> MAPVQLENHQLVPPGGGGGGSGGPPSAPAPPPPGAAVAAAAAAAASPGYRLSTLIEFLLHRAYSELMVLTDLLPRKSDVERKIEIVQFASRTRQLFVRLLALVKWANNAGKVEKCAMISSFLDQQAILFVDTADRLASLARDALVHARLPSFAIPYAIDVLTTGSYPRLPTCIRDKIIPPDPITKIEKQATLHQLNQILRHRLVTTDLPPQLANLTVANGRVKFRVEGEFEATLTVMGDDPDVPWRLLKLEILVEDKETGDGRALVHSMQISFIHQLVQSRLFADEKPLQDMYNCLHSFCLSLQLEVLHSQTLMLIRERWGDLVQVERYHAGKCLSLSVWNQQVLGRKTGTASVHKVTIKIDENDVSKPLQIFHDPPLPASDSKLVERAMKIDHLSIEKLLIDSVHARAHQKLQELKAILRGFNANENSSIETALPALVVPILEPCGNSECLHIFVDLHSGMFQLMLYGLDQATLDDMEKSVNDDMKRIIPWIQQLKFWLGQQRCKQSIKHLPTISSETLQLSNYSTHPIGNLSKNKLFIKLTRLPQYYIVVEMLEVPNKPTQLSYKYYFMSVNAADREDSPAMALLLQQFKENIQDLVFRTKTGKQTRTNAKRKLSDDPCPVESKKTKRAGEMCAFNKVLAHFVAMCDTNMPFVGLRLELSNLEIPHQGVQVEGDGFSHAIRLLKIPPCKGITEETQKALDRSLLDCTFRLQGRNNRTWVAELVFANCPLNGTSTREQGPSRHVYLTYENLLSEPVGGRKVVEMFLNDWNSIARLYECVLEFARSLPDIPAHLNIFSEVRVYNYRKLILCYGTTKGSSISIQWNSIHQKFHISLGTVGPNSGCSNCHNTILHQLQEMFNKTPNVVQLLQVLFDTQAPLNAINKLPTVPMLGLTQRTNTAYQCFSILPQSSTHIRLAFRNMYCIDIYCRSRGVVAIRDGAYSLFDNSKLVEGFYPAPGLKTFLNMFVDSNQDARRRSVNEDDNPPSPIGGDMMDSLISQLQPPPQQQPFPKQPGTSGAYPLTSPPTSYHSTVNQSPSMMHTQSPGNLHAASSPSGALRAPSPASFVPTPPPSSHGISIGPGASFASPHGTLDPSSPYTMVSPSGRAGNWPGSPQVSGPSPAARM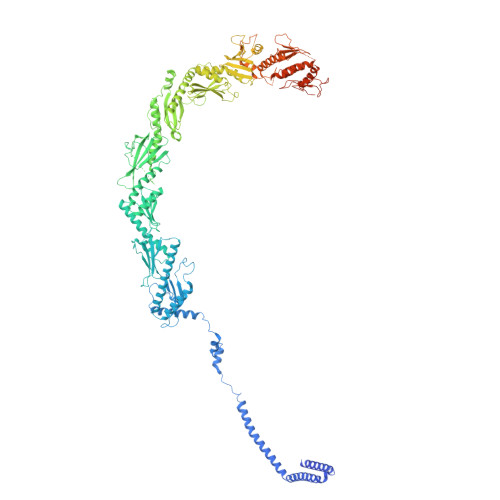PGMSPANPSLHSPVPDASHSPRAGTSSQTMPTNMPPPRKLPQRSWAASIPTILTHSALNILLLPSPTPGLVPGLAGSYLCSPLERFLGSVIMRRHLQRIIQQETLQLINSNEPGVIMFKTDALKCRVALSPKTNQTLQLKVTPENAGQWKPDELQVLEKFFETRVAGPPFKANTLIAFTKLLGAPTHILRDCVHIMKLELFPDQATQLKWNVQFCLTIPPSAPPIAPPGTPAVVLKSKMLFFLQLTQKTSVPPQEPVSIIVPIIYDMASGTTQQADIPRQQNSSVAAPMMVSNILKRFAEMNPPRQGECTIFAAVRDLMANLTLPPGGRP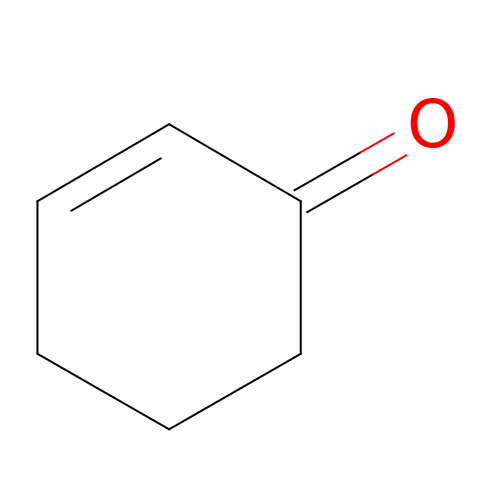cyclohex-2-en-1-one | C6 H8 O | FWFSEYBSWVRWGL-UHFFFAOYSA-N>[2x]KLATDIENNVRVVVYIRKDVEDNSQTIEKEGQTVTNNDYHKVYDSLKNMS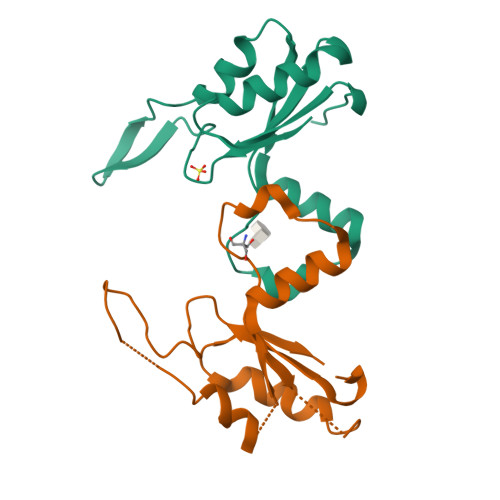TVKSVTFSSKEEQYEKLTEIMGDNWKIFEGDANPLYDAYIVEANAPNDVKTIAEDAKKIEGVSEVQD>MYSIEVRTHSALHVVKGAVVKVLGSEAKWTYSTYVKGNKGVLIVKFDRKPSDEEIREIERLANEKVKENAPIKIYELPR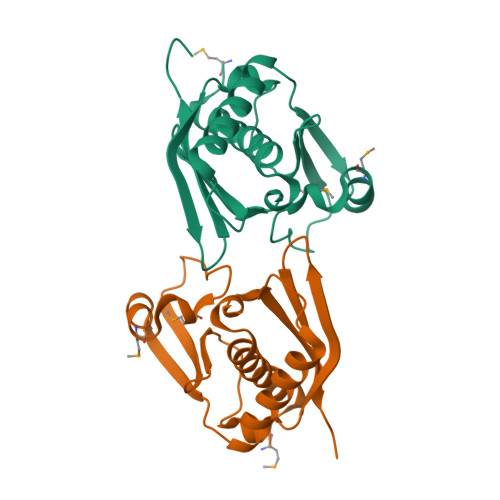EEAEKMFGEDMYDLFPVPEDVRILKVVVIEDWNVNACNKEHTKTTGEIGPIKIRKVRFRKSKGLLEIHFELLELENPSLEHHHHHH[2x]> GIDPFTMADDLPPAPVITAQASVPLTSESFVAAAVSRSGPAVVRIDTETVVTRRTDPILDDPFFQEFFGRSFPVPPRERRIAGQGSGFIIDNSGIILTNAHVVDGASKVVVTLRDGRTFDGQVRGTDEVTDLAVVKIEPQGSALPVAPLGTSSNLQVGDWAIAVGNPVGLDNTVTLGIISTLGRSAAQAGIPDKRVEFIQTDAAINPGNSGGPLLNAR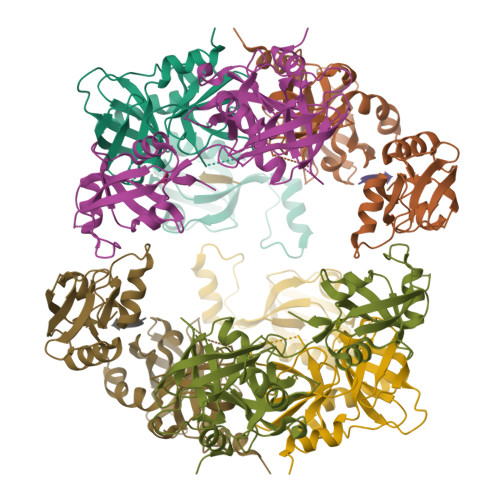GEVIGINTAIRADATGIGFAIPIDQAKAIQNTLAAGGTVPHPYIGVQMMNITVDQAQQNNRNPNSPFIIPEVDGILVMRVLPGTPAERAGIRRGDVIVAVDGTPISDGARLQRIVEQAGLNKALKLDLLRGDRRLSLTVQTAQLRNPTS;> AAAA> KEYDAYLSYTKVDQDTLDCDNPEEEQFALEVLPDVLEKHYGYKLFIPERDLIPSGTYMEDLTRYVEQSRRLIIVLTPDYILRRGWSIFELESRLHNMLVSGEIKVILIECTELKGKVNCQEVESLKRSIKLLSLIKWKGSKSSKLNSKFW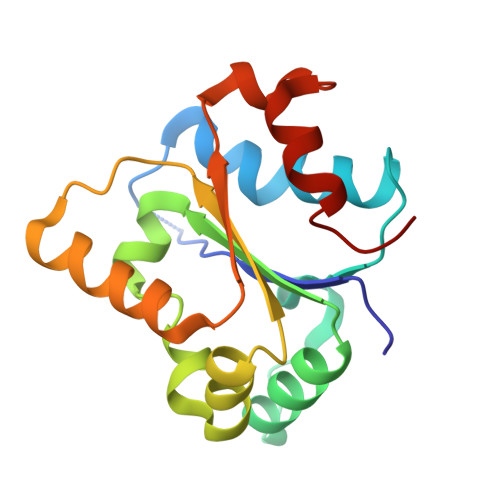KHLVYEMPIKK L-CARNITINYL-COA INNER SALT | C28 H49 N8 O18 P3 S | 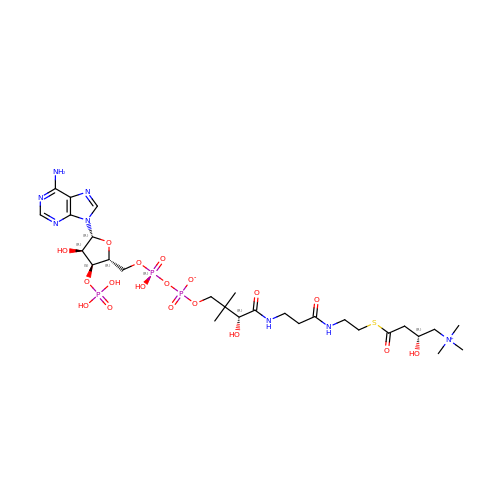BBRISSLDTUHWKG-PVMHLSDZSA-N Here, we present InCellCryst, an advanced pipeline for producing homogeneous microcrystals directly within living insect cells. We have demonstrated the pipeline on five different proteins (IMPDH, HEX-1, Cathepsin B, Luciferase and EGFP-µNS), representing a selection of soluble proteins of different source organisms that crystallize in insect cells in their native compartment or, in case of peroxisomes, readily in the cytoplasm or nucleus of the cells. Importantly, as shown for IMPDH and HEX-1, InCellCryst can produce crystals from native protein sequences, without purification tags or even remnants of proteolytically removed tags, within a quasi-native cellular environment. The rich source of biomolecules in the cellular environment allows the identification of native ligands by co-crystallization at quasi physiological conditions, representing a unique feature of InCellCryst.

All IMPDH structures show natural ligands at the canonical binding sites 1 and 2 in the Bateman domain. However, instead of guanosine monophosphate (GMP) found in the IMPDH N-His structure solved from isolated crystals, the structures solved in this study allow a clear identification of GDP in the canonical binding site 2, stabilized by hydrogen bonds to Lys133 and Arg101 that coordinate the α-phosphate and β-phosphate of GDP. In addition, a phosphate is bound to the IMP binding site of the catalytic domain of the IMPDH structures. As observed in the previously published IMPDH structure solved by SFX20, the canonical binding site 1 incorporates an ATP molecule. However, we observed two conformations of the bound ATP, where the gamma phosphates of the adjacent ATP molecules are either opposing or facing each other. The base and ribose are stabilized by interactions with Thr180, Thr174 or Asp158 and His200, whereas the different phosphate groups are interacting mainly with Thr156, Lys157, Arg219, Gly201, solvent molecules and the main chain. As shown here, serial synchrotron diffraction data can be processed by using CrystFEL and XDS. However, the identification of crystal wedges is a prerequisite for processing with XDS, which is mainly used for single crystal rotational datasets. Based on these results, in cellulo diffraction data collection clearly improves the bioinformation on natively bound ligands and their conformation compared to the diffraction of isolated in cellulo or conventionally grown crystals.

>[2x]MENTNLRTKTLRDGTTAEELFSQDGLSFNDFIILPGFIDFDSSKVNVSGQFTKNILLHLPLVSSPMDTVTESSMARAMALMGGIGVIHNNCTVEQQARMVRSVKLYRNGFIMKPKSVSPDVPVSTIRNIKSEKGISGILVTEGGKYDGKLLGIVCTKDIDFVKDASAPVSQYMTRRENMTVERYPIKLEEAMDVLNRSRHGYLPVLNDKDEVVCLCSRRDAVRARDYPNSSLDRNGHLLCAAATSTREADKGRVAALSEAGIDVLVLDSSQGNTIYQVSFIRWVKKTYPHLEVVAGNVVTQDQAKNLIDAGADSLRIGMGSGSICITQEVLACGRPQATAIYKVARYAASRGVPCVADGGLRNVGDVCKALAVGANVAMLGSMIAGTSETPGEYFFKDGMRLKGYRGMGSIDAMLQGRESGKRYLSENETLQVAQGVAGAVLDKGSVLKLLAYIHKGLQQSAQDIGEVSFDAIREKVYEGQVLFNRRSLTAQSEGAVHSLHHYERKLFASKL> RPQGATVSLWETVQKWREYRRQCQRSLTEDPPPATDLFCNRTFDEYACWPDGEPGSFVNVSCPWYLPWASSVPQGHVYRFCTAEGLWLQKDNSSLPWRDLSECEESKRGERSSP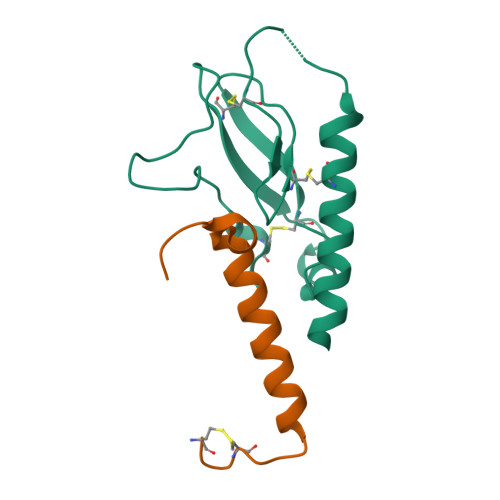EE;> HXEGXFTSDLSKQMEEEAVRLFIEWLKNGGPSSGAPPPS Ty3/Gypsy is a member of the Metaviridae family of LTR-retrotransposons characterised by a highly defined targeting pattern in S. cerevisiae, integrating in a narrow location 2–3 bp upstream of RNA Pol III-transcribed genes. The minimal factors required for Ty3 targeting at Pol III genes are the TFIIIB subunits, Brf1 and TBP, whereas TFIIIC is essential for directionality of integration, which occurs in a narrow window of 2–3 base pairs (bp) upstream the transcriptional start site (TSS). The Ty3 intasome is a pseudo-symmetrical tetrameric complex, in which the four integrase subunits are engaged with two Ty3 long-terminal repeats (LTR). Two “inner subunits” harbour the two active sites, placing in close juxtaposition the reactive LTR ends with the target DNA and are each associated with an outer subunit.

Following a process of hierarchical classification, we obtained a cryo-EM reconstruction of the Ty3 intasome engaged with TFIIIB and the target DNA at an overall resolution of 4.0 Å. Analysis of the structure reveals that a phosphodiester bond. has been formed between the 3’-end of the LTR reactive strands and a cleaved 5’-end on the target DNA, confirming the activity of the assembled complex and suggesting that the majority of the particles imaged by cryo-EM correspond to a strand-transfer complex. The integration reaction takes place at position −6 (relative to the TSS) of the non-template strand and position −2 (relative to the TSS) of the template strand, which would result in a 5 bp target site duplication (TSD) after a final step of DNA synthesis. Interaction of TFIIIB with the Ty3 intasome is mainly mediated by the C-terminal region of an outer Ty3 integrase subunit, which stablishes a novel set of contacts with the convex surface of TBP stirrups and Brf1 cyclin repeats. The SH3 fold (residues 369–433) of the CTD of an outer Ty3 subunit establishes direct protein–protein interactions with the H2’ helix of TBP C-terminal lobe, positioning the Ty3 intasome upstream the TSS. Topologically, this TBP-Ty3 interface overlaps with the binding interface of TBP and the RNA Pol II-specific transcription regulator negative cofactor 2 (NC2)49. The binding of TFIIIB far upstream (−15 to −32 bp) the TSS constrains the positioning of Ty3 intasome active site also upstream of the TSS, ensuring that RNA Pol III-transcribed genes are not disrupted by the integration event. The structural data unveils how a newly discovered chromodomain in Ty3 integrase mediates histone-independent interactions with Brf1 and the downstream part of the target DNA, acting as a “ruler” that safeguards the integration upstream of the transcription start site and prevents gene disruption.

>[4x]MSFMDQIPGGGNYPKLPVECLPNFPIQPSLTFRGRNDSHKLKNFISEIMLNMSMISWPNDASRIVYCRRHLLNPAAQWANDFVQEQGILEITFDTFIQGLYQHFYKPPDINKIFNAITQLSEAKLGIERLNQRFRKIWDRMPPDFMTEKAAIMTYTRLLTKETYNIVRMHKPETLKDAMEEAYQTTALTERFFPGFELDADGDTIIGATTHLQEEYDSDYDSEDNLTQNGYVHTVRTRRSYNKPMSNHRNRRNNNPSREECIKNRLCFYCKKEGHRLNECRARKAVLTDLELESKDQQTPFIKTLPIVHYIAIPEMDNTAEKTIKIQNTKVKTLFDSGSPTSFIRRDIVELLKYEIYETPPLRFRGFVATKSAVTSEAVTIDLKINDLHITLAAYILDNMDYQLLIGNPILRRYPKILHTVLNTRESPDSLKPKTYRSETVNNVRTYSAGNRGNPRNIKLSFAPTILEATDPKSAGNRGDSRTKTLSLATTTPAAIDPLTTLDNPGSTQSTFAQFPIPEEASILEEDGKYSNVVSTIQSVEPNATDHSNKDTFCTLPVWLQQKYREIIRNDLPPRPADINNIPVKHDIEIKPGARLPRLQPYHVTEKNEQEINKIVQKLLDNKFIVPSKSPCSSPVVLVPKKDGTFRLCVDYRTLNKATISDPFPLPRIDNLLSRIGNAQIFTTLDLHSGYHQIPMEPKDRYKTAFVTPSGKYEYTVMPFGLVNAPSTFARYMADTFRDLRFVNVYLDDILIFSESPEEHWKHLDTVLERLKNENLIVKKKKCKFASEETEFLGYSIGIQKIAPLQHKCAAIRDFPTPKTVKQAQRFLGMINYYRRFIPNCSKIAQPIQLFICDKSQWTEKQDKAIDKLKDALCNSPVLVPFNNKANYRLTTDASKDGIGAVLEEVDNKNKLVGVVGYFSKSLESAQKNYPAGELELLGIIKALHHFRYMLHGKHFTLRTDHISLLSLQNKNEPARRVQRWLDDLATYDFTLEYLAGPKNVVADAISRAVYTITPETSRPIDTESWKSYYKSDPLCSAVLIHMKELTQHNVTPEDMSAFRSYQKKLELSETFRKNYSLEDEMIYYQDRLVVPIKQQNAVMRLYHDHTLFGGHFGVTVTLAKISPIYYWPKLQHSIIQYIRTCVQCQLIKSHRPRLHGLLQPLPIAEGRWLDISMDFVTGLPPTSNNLNMILVVVDRFSKRAHFIATRKTLDATQLIDLLFRYIFSYHGFPRTITSDRDVRMTADKYQELTKRLGIKSTMSSANHPQTDGQSERTIQTLNRLLRAYASTNIQNWHVYLPQIEFVYNSTPTRTLGKSPFEIDLGYLPNTPAIKSDDEVNARSFTAVELAKHLKALTIQTKEQLEHAQIEMETNNNQRRKPLLLNIGDHVLVHRDAYFKKGAYMKVQQIYVGPFRVVKKINDNAYELDLNSHKKKHRVINVQFLKKFVYRPDAYPKNKPISSTERIKRAHEVTALIGIDTTHKTYLCHMQDVDPTLSVEYSEAEFCQIPERTRRSILANFRQLYETQDNPEREEDVVSQNEICQYDNTSP;> MSSIVNKSGTRFAPKVRQRRAATGGTPTPKPRTPQLFIPESKEIEEDNSDNDKGVDENETAIVEKPSLVGERSLEGFTLTGTNGHDNEIGDEGPIDASTQNPKADVIEDNVTLKPAPLQTHRDQKVPRSSRLASLSKDNESRPSFKPSFLDSSSNSNGTARRLSTISNKLPKKIRLGSITENDMNLKTFKRHRVLGKPSSAKKPAGAHRISIVSKISPPTAMTDSLDRNEFSSETSTSREADENENYVISKVKDIPKKVRDGESAKYFIDEENFTMAELCKPNFPIGQISENFEKSKMAKKAKLEKRRHLRELRMRARQEFKPLHSLTKEEQEEEEEKRKEERDKLLNADIPESDRKAHTAIQLKLNPDGTMAIDEETMVVDRHKNASIENEYKEKVDENPFANLYNYGSYGRGSYTDPWTVEEMIKFYKALSMWGTDFNLISQLYPYRSRKQVKAKFVNEEKKRPILIELALRSKLPPNFDEYCCEIKKNIGTVADFNEKLIELQNEHKHHMKEIEEAKNTAKEEDQTAQRLNDANLNKKGSGGIMTNDLKVYRKTEVVLGTIDDLKRKKLKERNNDDNEDNEGSEEEPEIDQ;> MADEERLKEFKEANKIVFDPNTRQVWENQNRDGTKPATTFQSEEDIKRAAPESEKDTSATSGIVPTLQNIVATVTLGCRLDLKTVALHARNAEYNPKRFAAVIMRIREPKTTALIFASGKMVVTGAKSEDDSKLASRKYARIIQKIGFAAKFTDFKIQNIVGSCDVKFPIRLEGLAFSHGTFSSYEPELFPGLIYRMVKPKIVLLIFVSGKIVLTGAKQREEIYQAFEAIYPVLSEFRKM;> MPVCKNCHGTEFERDLSNANNDLVCKACGVVSEDNPIVSEVTFGETSAGAAVVQGSFIGAGQSHAAFGGSSALESREATLNNARRKLRAVSYALHIPEYITDAAFQWYKLALANNFVQGRRSQNVIASCLYVACRKEKTHHMLIDFSSRLQVSVYSIGATFLKMVKKLHITELPLADPSLFIQHFAEKLDLADKKIKVVKDAVKLAQRMSKDWMFEGRRPAGIAGACILLACRMNNLRRTHTEIVAVSHVAEETLQQRLNEFKNTKAAKLSVQKFRENDVEDGEARPPSFVKNRKKERKIKDSLDKEEMFQTSEEALNKNPILTQVLGEQELSSKEVLFYLKQFSERRARVVERIKATNGIDGENIYHEGSENETRKRKLSEVSIQNEHVEGEDKETEGTEEKVKKVKTKTSEEKKENESGHFQDAIDGYSLETDPYCPRNLHLLPTTDTYLSKVSDDPDNLEDVDDEELNAHLLNEEASKLKERIWIGLNADFLLEQESKRLKQEADIATGNTSVKKKRTRRRNNTRSDEPTKTVDAAAAIGLMSDLQDKSGLHAALKAAEESGDFTTADSVKNMLQKASFSKKINYDAIDGLFR> SGEYTEIALPFSYDGAGEYYWKTDQFSTDPNDWSRYVNSWNLDLLEINGTDYTNVWVAQHQIPAA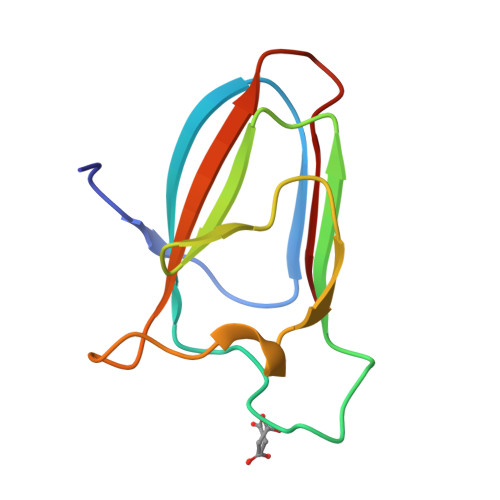SDGYWYIHYKSGVSWGHVEIK1-METHYL-5-(2-PHENOXYMETHYL-PYRROLIDINE-1-SULFONYL)-1H-INDOLE-2,3-DIONE | C20 H20 N2 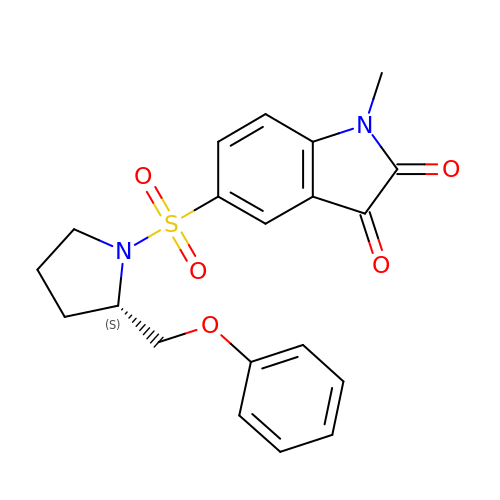O5 S | PFAYCUAUBOGVDX-AWEZNQCLSA-N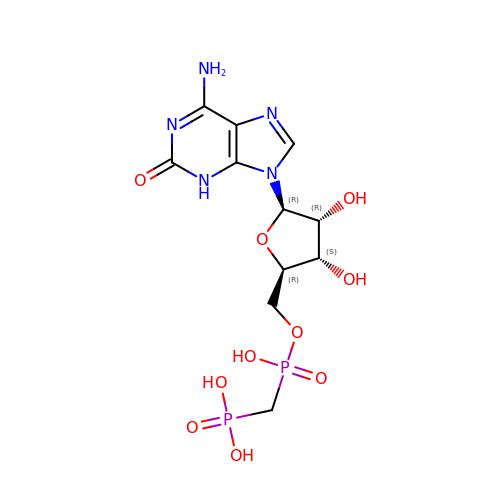[[(2~{R},3~{S},4~{R},5~{R})-5-(6-azanyl-2-oxidanylidene-3~{H}-purin-9-yl)-3,4-bis(oxidanyl)oxolan-2-yl]methoxy-oxidanyl-phosphoryl]methylphosphonic acid | C11 H17 N5 O10 P2 | ZFKXMQLZXNYUBT-KQYNXXCUSA-N> QTRHVKNYHSRSESTVENFLCRSACVFYTTYRNHGTDGDNFGYWVISTRQVAQLRRKLEMFTYARFDLELTFVITSTQEQSTIQGQDSPVLTHQIMYVPPGGPVPTKVNSYSWQTST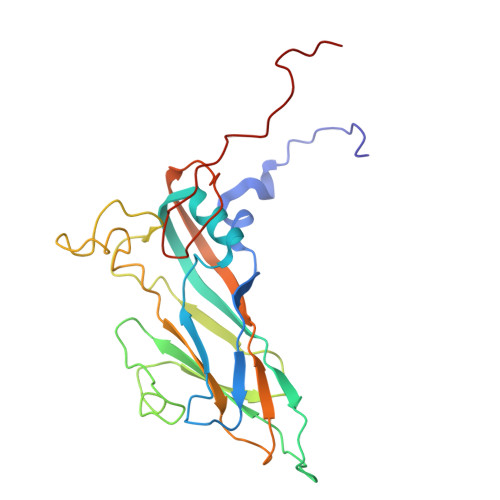NPSVFWTEGSAPPRMSIPFISIGNAYSMFYDGWAKFDKQGTYGINTLNNMGTLYMRHVNDGSPGPIVSTVRIYFKPKHVKTWVPRPPRLCQYQKAGNVNFEPTGVTESRTDITTMQ N-ethyl-N'-(5-methyl-1,2-oxazol-3-yl)urea | C7 H11 N3 O2 | 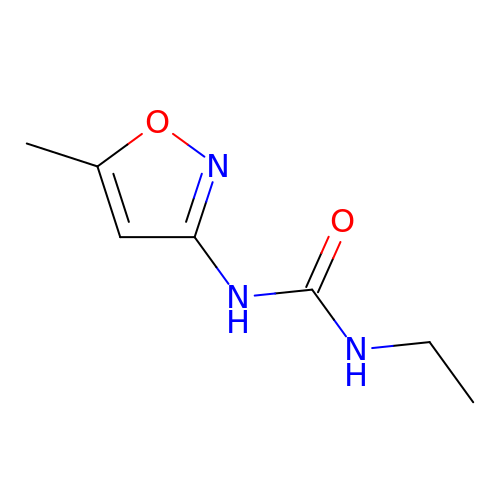OLTOJZGRSVNYRB-UHFFFAOYSA-N>[4x]EELIKENMHSKLYLEGSV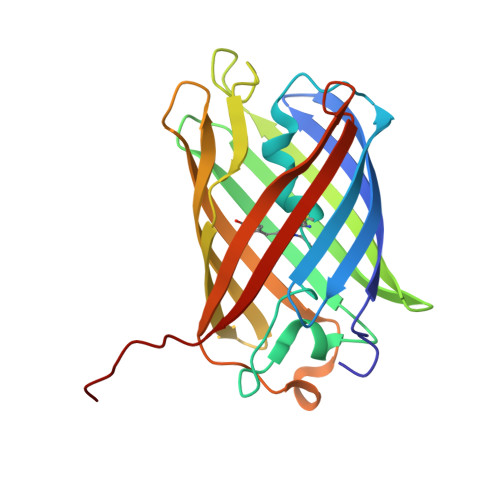NGHQFKCTHEGEGKPYEGTQTNRIKVVEGGPLPFAFDILATMFMYGSKAFIKYPKGLPDYFKQSFPEGFTWERTMVFEDGGVLTATQDTSLQDGCLIYNVKLRGVNFPANGPVMKQTTLGWEPSTETLYPADGALEGRCDMALKLVGGGHLHCNFKTTYKSKKPAKNLKMPGVHYVDRRLERIKEADNETYVEQHEVAVARYCDLPSKL>[2x]MAKKTSSLLSRRRTRRPGEPPLDLGSIPWLGYALDFGKDAASFLTRMKEKHGDIFTILVGGRYVTVLLDPHSYDAVVWEPRTRL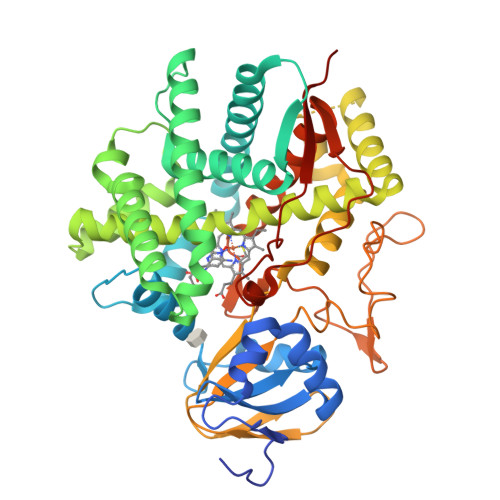DFHAYAIFLMERIFDVQLPHYSPSDEKARMKLTLLHRELQALTEAMYTNLHAVLLGDATEAGSGWHEMGLLDFSYSFLLRAGYLTLYGIEALPRTHESQAQDRVHSADVFHTFRQLDRLLPKLARGSLSVGDKDHMCSVKSRLWKLLSPARLARRAHRSKWLESYLLHLEEMGVSEEMQARALVLQLWATQGNMGPAAFWLLLFLLKNPEALAAVRGELESILWQAEQPVSQTTTLPQKVLDSTPVLDSVLSESLRLTAAPFITREVVVDLAMPMADGREFNLRRGDRLLLFPFLSPQRDPEIYTDPEVFKYNRFLNPDGSEKKDFYKDGKRLKNYNMPWGAGHNHCLGRSYAVNSIKQFVFLVLVHLDLELINADVEIPEFDLSRYGFGLMQPEHDVPVRYRIRPHHHHHHHH>MVLGKPQTDPTLEWFLSHCHIHKYPSKSTLIHQGEKAETLYYIVKGSVAVLIKDEEGKEMILFYLNQGDFIGELGLFEEGQERSAWVRAKTACEVAEISYKKFRQLIQVNPDILMRLSAQMARRLQVTSEKVGNLAFLDVTGRIAQTLLNLAKQPDAMTHPDGMQIKITRQEIGQIVGCSRETVGRILKMLEDQNLISAHGKT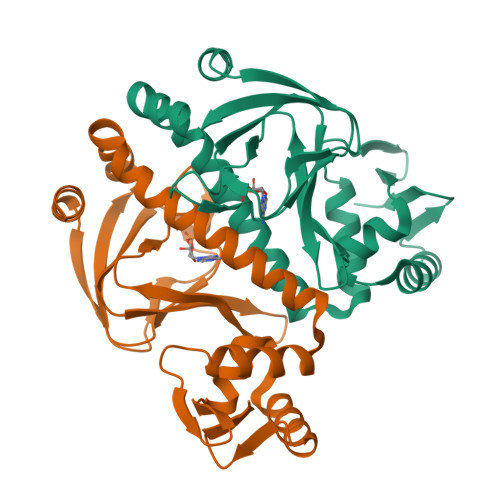IVVYGTR[2x]In Bacillus subtilis, the K+/H+ symporter KimA of the KUP family is inactivated by c-di-AMP. The c-di-AMP-sensitive, high-affinity K+/H+ symporter KimA from B. subtilis is particularly required for the uptake of potassium at low external potassium concentrations in acidic environments. As a member of the amino acid-polyamine-organocation (APC) superfamily it has the classical LeuT-fold with the first ten transmembrane helices (TMHs) adopting a 5 + 5 inverted repeat. KimA is a homodimer, stabilised by the swapping of the cytosolic domains with respect to the transmembrane domain.

KimA in DDM was additionally incubated with a ten-fold molar excess of c-di-AMP after purification. The overall structure of KimA obtained from the preparation in DDM resembles the previous structure obtained in SMALPs25 (RMSDs of TMD (residues 30–462): 1.31 Å, CD (residues 462–606): 1.65 Å, global RMSD: 1.74 Å). The two TMDs are tilted towards each other, forming a dimer interface at the extracellular side that would enforce a bending of the membrane by ~130° against its natural curvature. As speculated for the preparation of KimA in SMALPs, the tilting likely was caused by a loss of lipids between the TMDs during purification. A comparison of the resulting structures of KimA in DDM and in amphipols with the previously reported structure from SMALPs25 suggests that all of them represent a similar inward-occluded conformation. In agreement with this, a strong density for the bound substrate potassium ion is observed in the 3.3 Å cryo-EM map. The potassium ion is coordinated by Tyr43 (2.9 Å), the carbonyl and carboxyl of Asp36 (2.8 Å and 3.3 Å, respectively), hydroxyl and carbonyl of Thr230 (2.9 and 3.2 Å, respectively) and Tyr377 (3.2 Å). Each binding site is formed mostly by the cytosolic domain of one monomer: One of the phosphodiesters of c-di-AMP is coordinated through two hydrogen bonds and a salt bridge between the non-esterified oxygen atoms and the amide groups of Gln581 and Ser582 and the guanidinium group of Arg337. Only the second adenosine moiety is coordinated by residues of the neighbouring protomer; it is stacked between Val457 and Leu461 of TMH 12 that extends out of the membrane and Arg337, located in the loop between TMHs 8 and 9. Arg337 is the only residue of the TMD that engages in a strong interaction with c-di-AMP, making it a prime candidate for the transmission of the inhibitory effect of bound c-di-AMP.

>MYHSIKRFLIGKPLKSQAAGEQKLTKLKALAMLSSDALSSVAYGTEQILIILATISAAAFWYSIPIAVGVLILLLALILSYRQIIYAYPQGGGAYIVSKENLGEKPGLIAGGSLLVDYILTVAVSISAGTDAITSAFPALHDYHVPIAIFLVLVIMILNLRGLSESASILAYPVYLFVVALLVLIAVGLFKLMTGQIDQPAHHTSLGTPVAGITLFLLLKAFSSGCSALTGVEAISNAIPAFKNPPARNAARTLAMMGILLAILFSGITVLAYGYGTAPKPDETVVSQIASETFGRNVFYYVIQGVTSLILVLAANTGFSAFPQLAFNLARDQYMPRMFTVRGDRLGFSNGIIFLGFASIVLIILFGGQTEHLIPLYAVGVFIPFTLSQTGMCMKWIKQKPKGWIGKMLINSCGALISFMVLSILFVTKFNVVWPVLIFMPIVVLLFFAIKNHYTAVGEQLRIVDKEPEEIKGTVVIVPVAGVTTVVQKSIHYAKSLSDQVIAVHVSFDREQEKKFEKRWEELNNGVRLVTLHSSYRSLVHPFDKFLETVEAKAKKEQFSVMVLFPQFITKKRWHTILHNQSAFLLRVRLFWKKDIMVATLPYHFKK[2x]> MPSELTPEERSELKNSIAEFHTYQLDPGSCSSLHAQRIH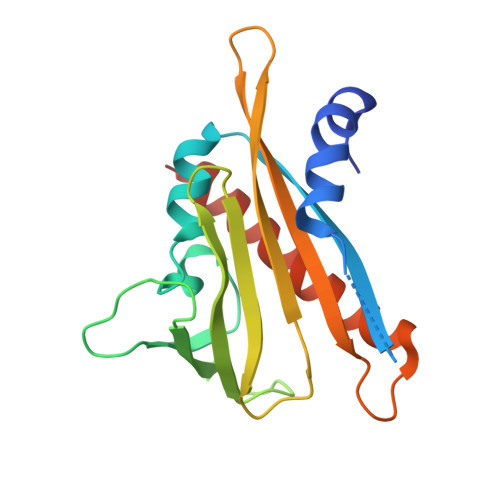APPELVWSIVRRFDKPQTHRHFIKSCSVEQNFEMRVGCTRDIIVISGLPANTSTERLDILDDERRVTGASIIGGEHRLTNYKGVTTVHRFEKENRIWTVVLESYVVDMPEGNSEDDTRIVVDDVVKLNLQKLATVAEAMARN> MSQASLREGAAGELQLAGVLDYSSGPALREQGGRLIRASQAAELVVDCSAVERSSSVGISLLLAFIRDARKAGKVLSVRALPDDMREIAKVS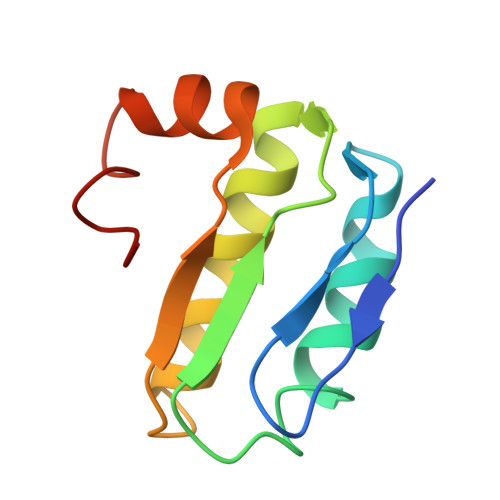SLLEILPLQE>[6x]MRGSHHHHHHGSMPVAGSELPRRPLPPAAQERDAEPRPPHGELQYLGQIQHILRCGVRKDDRTGTGTLSVFGMQARYSLRDEFPLLTTKRVFWKGVLEELLWFIKGSTNAKELSSKGVKIWDANGSRDFLDSLGFSTREEGDLGPVYGFQWRHFGAEYRDMESDYSGQGVDQLQRVIDTIKTNPDDRRIIMCAWNPRDLPLMALPPCHALCQFYVVNSELSCQLYQRSGDMGLGVPFNIASYALLTYMIAHITGLKPGDFIHTLGDAHIYLNHIEPLKIQLQREPRPFPKLRILRKVEKIDDFKAEDFQIEGYNPHPTIKMEMAV

Human thymidylate synthase adopts two different conformations, named active and inactive, that equilibrate with each other. The equilibrium position depends on mutations, on binding of substrates/substrate analogs/inhibitors either in the active site cavity or at the dimer interface, and on crystallization conditions. 5FU and RTX are both used in chemotherapy against solid cancers. They inhibit hTS by targeting the enzyme active site. While FdUMP competes with the substrate, dUMP (2′-deoxyuridine-5′-monophosphate), RTX competes with the cofactor, N5, N10-methylenetatrahydrofolate (mTHF).

The present crystal structure of the hTS:FdUMP:RTX complex shows six independent enzyme subunits arranged in three homodimers in the triclinic unit cell. All six subunits are in the active conformation and host in the active site one FdUMP and one RTX molecule. In particular, FdUMP occupies the same binding site as the natural substrate, dUMP, and is at contact distance with the catalytic Cys195. In the hTS:dUMP/FdUMP:RTX ternary complexes, the phosphate group of FdUMP is bound in the same way as the dUMP phosphate; RMSD upon superimposition of the two structures showed only minor changes at the interface of the two subunits where it engages salt links with four arginine residues belonging to both dimer halves (Arg50 and Arg250 from one subunit and Arg175′ and Arg176′ from the facing protomer), and a H-bond with the side chain of Ser216. A double H-bond bridge, reminiscent of the nucleic acid base pairs, links the FdUMP pyrimidine N3 and O4 atoms to Asn226 Nδ2 and Oδ1, respectively. The fluorine atom of FdUMP is within contact distance (3.6–4.0 Å) from the side chain of Trp109 while it does not interact with the side chain of the catalytic Cys195 that points away from it. RTX, besides giving the mentioned stacking interactions with FdUMP, is involved in few H-bonds with the enzyme: the quinazoline N3 and O4 atoms are H-bonded to the Asp218 side chain and to the NH of Gly222 respectively. The RTX terminal glutamic acid displays weak electron density and appears disordered and in different conformations. However, no covalent bond between the protein and the nucleotide is found in the X-ray crystal structure of the hTS:FdUMP:RTX ternary complex. The existence of the attractive stacking interactions between the pyrimidine and quinazoline rings and the absence of hindering interactions between the two bound inhibitors lead to a stabilization of the active complex.>SNAMRDYTKQYINGEWVESNSNETIEVINPATEEVIGKVAKGNKADVDKAVEAADDVYLEFRHTSVKERQALLDKIVKEYENRKDDIVQAITDELGAPLSLSERVHYQMGLNHFVAARDALDNYEFEERRGDDLVVKEAIGVSGLITPWNFPTNQTSLKLAAAFAAGSPVVLKPSEETPFAAVILAEIFDKVGVPKGVFNLVNGDGAGVGNPLSEHPKVRMMSFTGSGPTGSKIMEKAAKDFKKVSLELGGKSPYIVLDDVDIKEAAKATTGKVVNNTGQVCTAGTRVLVPNKIKDAFLAELKEQFSQVRVGNPREDGTQVGPIISKKQFDQVQNYINKGIEEGAELFYGGPGKPEGLEKGYFARPTIFINVDNQMTIAQEEIFGPVMSVITYNDLDEAIQIANDTKYGLAGYVIGKDKETLHKVARSIEAGTVEINEAGRKPDLPF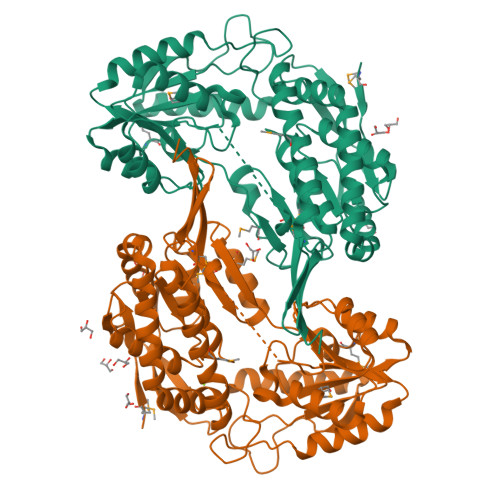GGYKQSGLGREWGDYGIEEFLEVKSIAGYFK[2x]> LYHTVPPAVVGVGGGGVNAGPVASGAIVGTNGYVITTLHSVSKLPEISVQVATTGGIRRFPAQVVKTIPGHDLALLKMQTTEKFLHFRMADVQTVVPGQQVFAFGRNMAGAPLVRQGLVQSADAPLAVGATQITHLLRSDAVYSWEQTGGPLVN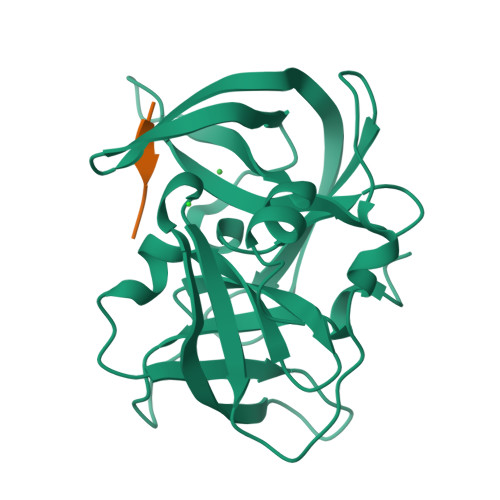AQGDLVGINIAATGPTGKVEGFTVPAQVIVSHLQDVV>GSFIDIEFPEWFHEGLSRHQAENLLMGKDIGFFIIRASQSSPGDFSISVRHEDDVQHFKVMRDTKGNYFLWTEKFPSLNKL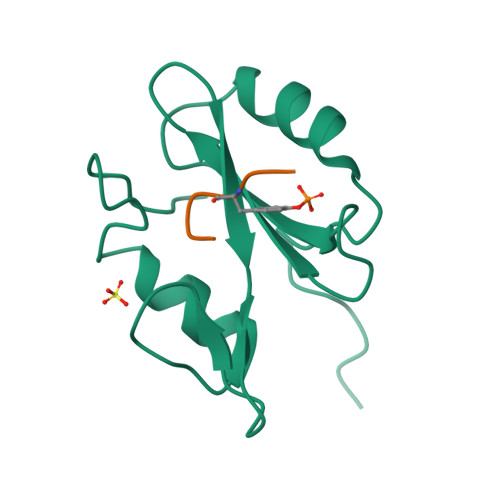VDYYRTTSISKQKQVFLRD[2x];>XREYVNV[2x]> GMYEEWKIVKREAPILGNDQLIENIWKMKREDSPYDIISL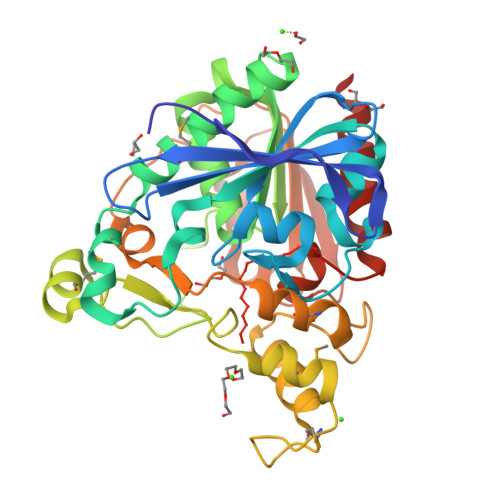HKVNLIGGGNDAVLILPGTWSSGEQLVTISWNGVHYTIPDYRKSIVLYLARNGFNVYTIDYRTHYVPPFLKDRQLSFTANWGWSTWISDIKEVVSFIKRDSGQERIYLAGESFGGIAALNYSSLYWKNDIKGLILLDGGPTKHGIRPKFYTPEVNSIEEMEAKGIYVIPSRGGPNNPIWSYALANPDMPSPDPKYKSISDFLMDSLYVTGSANPYDYPYSKKEDMFPILASFDPYWPYRLSLERDLKFDYEGILVPTIAFVSERFGIQIFDSKILPSNSEIILLKGYGHLDVYTGENSEKDVNSVVLKWLSQQR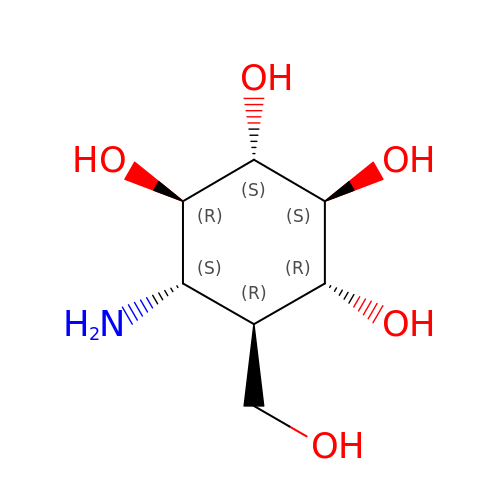(1R,2S,3S,4R,5S,6R)-5-amino-6-(hydroxymethyl)cyclohexane-1,2,3,4-tetrol | C7 H15 N O5 | SWVTZDDSAFUTKS-DBTJYCMPSA-N> GDVEEAIDRAVARVADTMPTGPRNTESVPALTAVETGHTSQVVPGDTMQTRHVKNYHSRTESSIENFLCRAACVYIATYKSAGGTPTERYASWRINTRQMVQLRRKFELFTYLRFDMEITFVITSTQDPGTQLAQDMPVLTHQIMYIPPGGPVPNSATDFAWQSSTNPSIFWTEGCAPARMSVPFISIGNAYSNFYDGWSHFTQEGVYGFNSLNNMGHIYVRHVNEQSLGVSTSTLRVYFKPKHVRAWVPRPPRLSPYVKSSNVNFKPTAVTTERKDINDVGT;> SPTVEECGFSDRVRSITLGNSTITTQECANVVVGYGVWPSYLQDNEATAEDQPTQPDVATCRFYTLDSIQWQKESDGWWWKFPEALKNMGLFGQNMEYHYLGRSGYTIHVQCNASKFHQGCLLVVCVPEAEMGCSDVEREVVAASLSSEDTAKSFSRTESNGQHTVQTVVYNAGMGVGVGNLTIFPHQWINLRTNNSATIVMPYINSVPMDNMFRHYNFTLMIIPFAKLEYTEQASNYVPITVTVAPMCAEYNGLRLASHQ;> GLPTMLTPGSNQFLTSDDFQSPSAMPQFDVTPEMKIPGEVHNLMEIAEVDSVVPVNNTKENINSMEAYRIPVTGGDQLHTQVFGFQMQPGLNSVFKRTLLGEILNYYAHWSGSVKLTFVFCGSAMATGKFLLAYSPPGASPPQNRKQAMLGTHVIWDVGLQSSCVLCIPWISQTHYRLVQQDE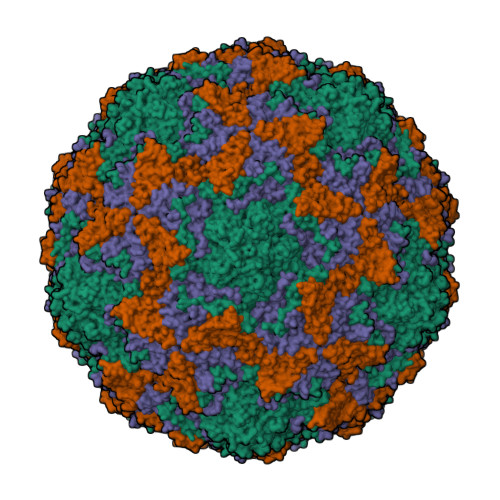YTSAGYVTCWYQTGLIVPPGAPPSCTILCFASACNDFSVRMLRDTPFIEQTQLLQ;> GAQVSTQKTGAHETSLTASGNSTIHYTNINYYKDAASNSANRQDFTQDPSKFTEPMKDVMIKSLPALN> MHPETLVKVKDAEDQLGARVGYIELDLNSGKILESFRPEERFPMMSTFKVLLCGAVLSRIDAGQEQLGRRIHYSQNDLVEYSPVTEKHLTDGMTVRELCSAAITMSDNTAANLLLTTIGGPKELTAFLHNMGDHVTRLDRWEPELNEAIPNDERDTTMPAAMATTLRKLLTGELLTLASRQQLIDWMEADKVAGPLLRSALPAGWFIADKSGAGERGSRGIIAALGPDGKPSRIVVIYTTGSQATMDERNRQIAEIGASLIKHW;> AHPETLVKVKDAKDQLGKRVGYIELDLASGKILVSFRPEERFPMMSTFKVLLCGAVLSRVDAGQEQLGRRIHYSQNDLVEYSPVTEKHLTDGMTVGELCSAAITMSDNTAANLLLTTIGGPKELTAFLHNMGDHVTR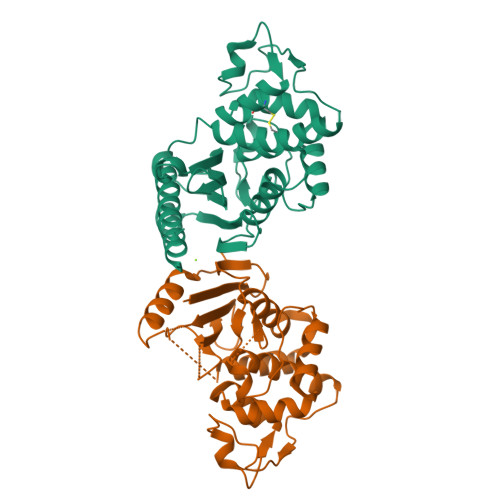LDRWEPELNEAIPNDERDTTTPVAMATTLRKLLTGELLTAASRQQLIDWMEADKVAGPLLRSALPAGWFIADKSGAGERGSRGIIAALGPDGKPSRIVVIYMTGSQATMDERNRQIAEIGASLIKHWA> MASIWVGHRGTVRDYPDFSPSVDAEAIQKAIRGIGTDEKMLISILTERSNAQRQLIVKEYQAAYGKELKDDLKGDLSGHFEHLMVALVTPPAVFDAKQLKKSMKGAGTNEDALIEILTTRTSRQMKDISQAYYTVYKKSLGDDISSETSGDFRKALLTLADGRRDESLKVDEHLAKQDAQILYKAGENRWGTDE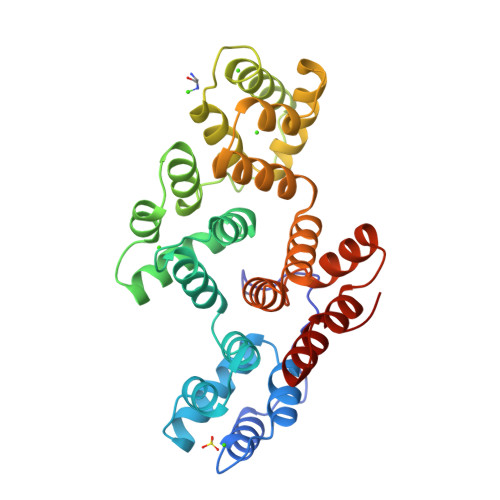DKFTEILCLRSFPQLKLTFDEYRNISQKDIVDSIKGELSGHFEDLLLAIVNCVRNTPAFLAERLHRALKGIGTDEFTLNRIMVSRSEIDLLDIRTEFKKHYGYSLYSAIKSDTSGDYEITLLKICGGDD4-{(2E)-3-[4-{[2-(pyridin-3-ylmethoxy)phenyl]sulfanyl}-2,3-bis(trifluoromethyl)phenyl]prop-2-enoyl}morpholine 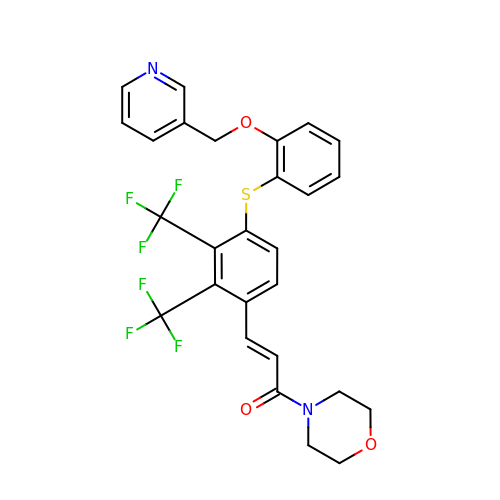| C27 H22 F6 N2 O3 S | ZRIKDHLPCRURPX-CSKARUKUSA-N> AGAGAAIAUCU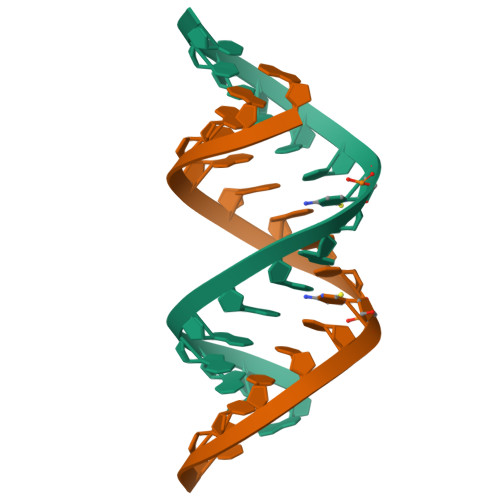UCUCU>KVVAKGLGLSKAYVGQKSSFTVDCSKAGNNMLLVGVHGPRTPCEEILVKHVGSRLYSVSYLLKDKGEYTLVVKWG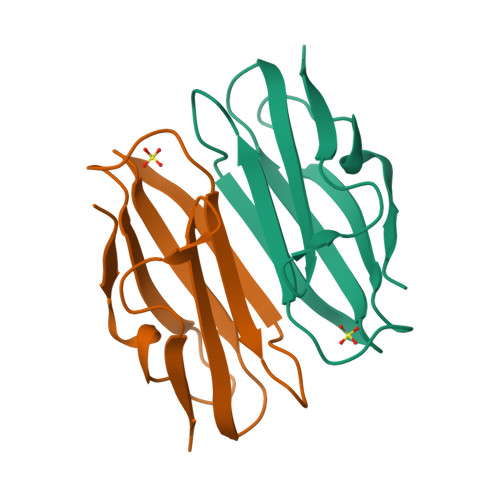HEHIPGSPYRVVVP[2x]Interestingly, the type I-D system utilizes subunits that are homologs of type I complexes, type III complexes, or both. The type I-D operon contains the type I signature gene cas3 split into its two domains; the helicase domain (Cas3′) encoded from a stand-alone gene, and the HD nuclease domain (Cas3″), which is fused to the large subunit as part of the core effector complex. The Cas10d subunit is bigger than other type I large subunits (Cas8) and similar to type III large subunits, yet retains the type I functionality of discerning PAMs in target DNA sequences. As is typical for Cascade complexes, a repeating, helical backbone of Cas7d subunits assembles around the crRNA, while the C-terminus of Cas10d and two Cas11d subunits constitute a minor filament along the belly of the complex.

To obtain mechanistic insight into dsDNA targeting, we employed cryo-electron microscopy to directly visualize type I-D Cascade bound to dsDNA with a protospacer sequence complementary to the crRNA and flanked by a GTT PAM. We employed focused 3D classification to overcome local conformational heterogeneity, which yielded a structure of the dsDNA-bound type I-D Cascade at a global resolution of 2.9 Å and enabled de novo atomic modeling of the entire complex. The stoichiometry of the complex was Cas10d1:Cas7d7:Cas5d1:Cas11d2, highlighting the addition of one Cas7d subunit compared to our recent sub-nanometer structure. We resolved 43 bases of the crRNA scaffold in the Cascade-dsDNA complex, as well as 16 bases of the target strand (TS) and 13 bases (five of which we modeled as poly-T) of the non-target strand (NTS). The unwinding of the dsDNA duplex occurs between a cleft created by the bottom Cas7 subunit and the spur on Cas10d, which we assign as the PAM-recognition domain (PRD). At the DNA duplex PAM site, we observe a loop from Cas10d wedged into the minor groove of the PAM duplex. One glycine (G433) interacts with the G (−3 position) in the NTS of the PAM, providing an anchor for the loop to lock into the minor groove. The K326 residue in Cas10d recognizes the C (−3 position) on the TS, the T (−2 position) on the NTS, and the G (−3 position) on the NTS via hydrogen bonding. In comparison to the ssRNA target-bound complex, the dsDNA-bound complex undergoes a continuous 5 Å shift of the small subunits away from the belly of the complex and slightly downwards towards Cas10d, along with a similar shift of Cas10d downwards.

>[7x]MLDSLKSQFQPSFPRLASGHYVHFLMLRHSQSFPVFQTDGVLNTTRTQAGLLEKTDQLSRLVMFKRKQTTPERLAGRELLRNLGLTSADKSAKNLCEYNGEGSCKQCPDCILYGFAIGDSGSERSKVYSDSAFSLGAYEQSHRSFTFNAPFEGGTMSEAGVMRSAINELDHILPEVTFPTVESLRDATYEGFIYVLGNLLRTKRYGAQESRTGTMKNHLVGIVFADGEIFSNLHLTQALYDQMGGELNKPISELCETAATVAQDLLNKEPVRKSELIFGAHLDTLLQEVNDIYQNDAELTKLLGSLYQQTQDYATEFGALSGGKKKAKS;> MTKIYRCKLTLHDNVFFASREMGILYETEKYFHNWALSYAFFKGTIIPHPYGLVGQNAQTPAYLDRDREQNLLHLNDSGIYVFPAQPIHWSYQINTFKAAQSAYYGRSVQFGGKGATKNYPINYGRAKELAVGSEFLTYIVSQKELDLPVWIRLGKWSSKIRVEVEAIAPDQIKTASGVYVCNHPLNPLDCPANQQILLYNRVVMPPSSLFSQSQLQGDYWQIDRNTFLPQGFHYGATTAIAQDSPQLSLLDTN;> MTTLLQTLLIRTLSEQKDYILLEYFQTILPALEEHFGNTSGLGGSFISHQKHFGTQGYDTEKAKKMAQGFAKKGDQTLAAHILNALLTTWNVMQELEFPLNDIERRLLCLGITLHDYDKHCHAQDMAAPEPDNIQEIINICLELGKRLNFDEFWADWRDYIAEISYLAQNTHGKQHTNLISSNWSNAGYPFTIKERKLDHPLRHLLTFGDVAVHLSSPHDLVSSTMGDRLRDLLNRLGIEKRFVYHHLRDTTGILSNAIHNVILRTVQKLDWKPLLFFAQGVIYFAPQDTEIPERNEIKQIVWQGISQELGKKMSAGDVGFKRDGKGLKVSPQTSELLAAADIVRILPQVISVKVNNAKSPATPKRLEKLELGDAEREKLYEVADLRCDRLAELLGLVQKEIFLLPEPFIEWVLKDLELTSVIMPEETQVQSGGVNYGWYRVAAHYVANHATWDLEEFQEFLQGFGDRLATWAEEEGYFAEHQSPTRQIFEDYLDRYLEIQGWESDHQAFIQELENYVNAKTKKSKQPICSLSSGEFPSEDQMDSVVLFKPQQYSNKNPLGGGQIKRGISKIWSLEMLLRQAFWSVPSGKFEDQQPIFIYLYPAYVYAPQVVEAIRELVYGIASVNLWDVRKHWVNNKMDLTSLKSLPWLNEEVEAGTNAQLKYTKEDLPFLATVYTTTREKTDTDAWVKPAFLALLLPYLLGVKAIATRSMVPLYRSDQDFRESIHLDGVAGFWSLLGIPTDLRVEDITPALNKLLAIYTLHLAARSSPPKARWQDLPKTVQEVMTDVLNVFALAEQGLRREKRDRPYESEVTEYWQFAELFSQGNIVMTEKLKLTKRLVEEYRRFYQVELSKKPSTHAILLPLSKALEQILSVPDDWDEEELILQGSGQLQAALDRQEVYTRPIIKDKSVAYETRQLQELEAIQIFMTTCVRDLFGEMCKGDRAILQEQRNRIKSGAEFAYRLLALEAQQNQN;>MTEKLKLTKRLVEEYRRFYQVELSKKPSTHAILLPLSKALEQILSVPDDWDEEELILQGSGQLQAALDRQEVYTRPIIKDKSVAYETRQLQELEAIQIFMTTCVRDLFGEMCKGDRAILQEQRNRIKSGAEFAYRLLALEAQQNQN[2x]>SNATIYRMVDLPVIQPRLCTHARWPAPVYGLLVDPSLPSNPQWQNGRVHVDGTLLGTTPISGSWVSCFAAEAAYEFQSGTGEVATFTLIEQDGSAYVPGDRAAPLGYPDFSGQLEIEVQTETTKTGDKLKVTTFEMILGPTTNADQAPYQGRVFASVTAAASLDLVDGRVRA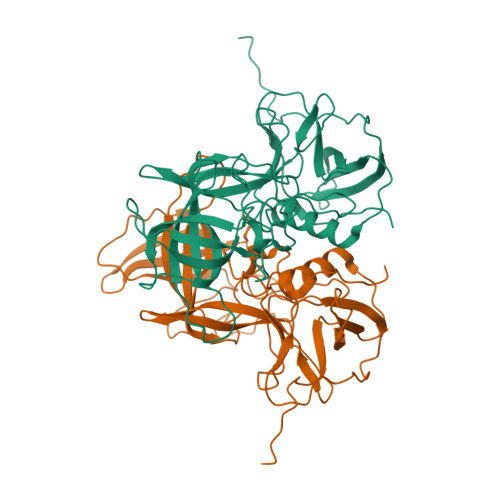VPRSIYGFQDTIPEYNDGLLVPLAPPIGPFLPGEVLLRFRTYMRQIDTADAAAEAIDCALPQEFVSWFASNAFTVQSEALLLRYRNTLTGQLLFECKLYNEGYIALSYSGSGPLTFPTDGIFEVVSWVPRLYQLASVGSLATGRMLKQ[2x]> MIWKYLQRTNRGNIIQAGLQHRKFENLPFKQNFDNLTKAYDLRMWYISNSPHEAKNLEYVNELEALHNELNYQNSRQ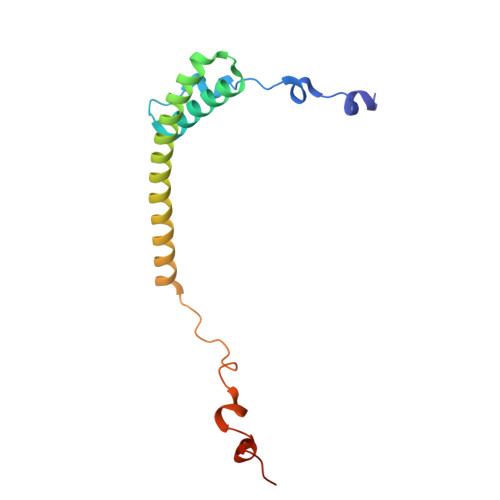FLFRTVSFLLGWALFYQFYELPKTYDWQDTQEPKHQVPAYGDLEEGGDEGGDD> MAVRASEISRVYEAYPEKKATLYFLVLGFLALIVGSLFGPFQALNYGNVDAYPLLKRLLPFVQSYYQGLTLHGVLNAIVFTQLFAQAIMVYLPARELNMRPNMGLMWLSWWMAFIGLVVAALPLLANEATVLYTFYPPLKGHWAFYLGASVFVLSTWVSIYIVLDLWRRWKAANPGKVTPLVTYMAVVFWLMWFLASLGLVLEAVLFLLPWSFGLVEGVDPLV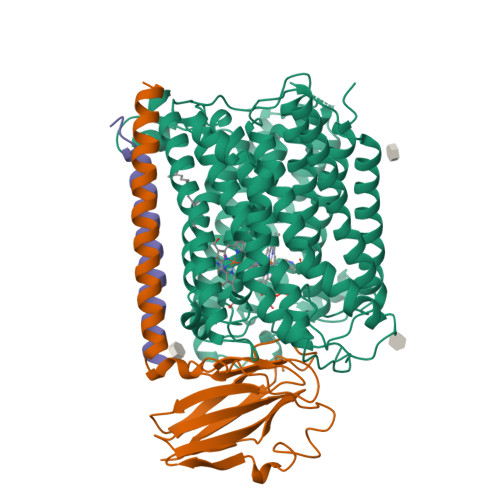ARTLFWWTGHPIVYFWLLPAYAIIYTILPKQAGGKLVSDPMARLAFLLFLLLSTPVGFHHQFADPGIDPTWKMIHSVLTLFVAVPSLMTAFTVAASLEFAGRLRGGRGLFGWIRALPWDNPAFVAPVLGLLGFIPGGAGGIVNASFTLDYVVHNTAWVPGHFHLQVASLVTLTAMGSLYWLLPNLTGKPISDAQRRLGLAVVWLWFLGMMIMAVGLHWAGLLNVPRRAYIAQVPDAYPHAAVPMVFNVLAGIVLLVALLLFIYGLFSVLLSRERKPELAEAPLPFAEVISGPEDRRLVLAMDRIGFWFAVAAILVVLAYGPTLVQLFGHLNPVPGWRLW;> MVDEHKAHKAILAYEKGWLAFSLAMLFVFIALIAYTLATHTAGVIPAGKLERVDPTTVRQEGPWADPAQAVVQTGPNQYTVYVLAFAFGYQPNPIEVPQGAEIVFKITSPDVIHGFHVEGTNINVEVLPGEVSTVRYTFKRPGEYRIICNQYCGLGHQNMFGTIVVKE;> EEKPKGALAVILVLTLTILVFWLGVYAVFFARG The assembly of the mitoribosomal small subunit involves folding and modification of rRNA, and its association with mitoribosomal proteins. This process is assisted by a dynamic network of assembly factors. Conserved methyltransferases Mettl15 and Mettl17 act on the solvent-exposed surface of rRNA. Mettl15 is a class I SAM-dependent N4-methylcytidine (m4C) methyltransferase of bacterial origin that modifies the mtSSU rRNA at position C1486 (human numbering).

Using the data from recently published structures of mammalian pre-mitoribosomal intermediates, we analysed the T. brucei maps and identified a number of previously undescribed structural elements. First, we detected homologs of RbfA and Mettl15 (previously referred to as mt-SAF18 and mt-SAF14, respectively), both of which are associated with Mettl17 (mt-SAF1). Structurally, RbfA is anchored to the complex by its N-terminal extension, with the C-terminal domain binding Mettl17 and the C-terminal extension binding Mettl15. Together, these elements stabilize the subcomplex in a way that Mettl15 and Mettl17 form a heterodimer that is bound in the cleft between the head and body. In total there are 43 hydrogen bonds and ten salt bridges that stabilize the Mettl15-Mettl17 heterodimer, which contribute to two main interfaces. The second interface involves catalytic domains of both Mettl17 and Mettl15 (residues 484–512 and 176–198, respectively). These data suggest that in T. brucei Mettl15 and Mettl17 form a stable complex, which has not been observed in other species. In Mettl15, SAM is located 42 Å away from the methyltransferase target residue cytidine 582 (C582, equivalent of human C1486), implying a non-catalytic conformation. The Mettl15 conformation is different from that observed in the mammalian m4C1486-containing post-catalytic precursor, thus implying a pre-catalytic state. Finally, we identified 13 hammerhead-shaped densities ranging from 17 to 22 Å in length, coordinated by tryptophan residues within a helix-loop-helix motif of pentatricopeptide repeat (PPR) proteins, which likely represent cofactors such as acetyl coenzyme A (acetyl-CoA).

> MFLIHFVHYKTILQKYTFKFKHIFLSIDKYNSLFFNISGILIWLNIIHINIILIKYSFFILINNFEYLIILIST;> MFRLTAASQKNLNSWYTKGTMRGGVPRIYYAWMRPGSFTRRRFEKMRNPFVDLETGTSLYFRDTRDSAEAIAHAADSKGIKGMDNAIDLYNEYRIVPDLYPEGFQWKHKLNTEYNQWRSNTWLTPDLIPKEHRGRFLCNFQLNIVAYDMRVVKFSPKDHRQWIYCVLYVGSGKGIAGWGRAVAPSTQEAKKEAIREAFSNIIAVDLEQEGPMYPVRVNADGVRVLLYPARRIVANFRVADILCAFGFQHAGCRINLKATNNPKSPTHTVEGVFEAVKALRSVSEIAASRGKVPHSLIYNIYPYLEEIRRRKGMMAMHPPGKDGLLMPDRVVDNRLPDHLKKGYYDDVYWKDFFAGSDEHLNEPRMGLRGDEMRRRLEEAQTSPAPTTAKDTRRRTLEDVLKRLGKTTRDLGSIPIVNPRVDVGLPTHIKRNYQLH;> MVFYSFVLVMKPRQRRFTSQALREIGVAVYSNGGLIRSITNEGIMRPYSRFRDADNTPLTYARYIILQLDMGEEEMGKVDKIIREHQDVLMALKLNNLERPVGIRSGNKELQAAYFPLDTFTRLEEEINWSPQTSADIYTQLEMNWKEFSRTRWSSFLRN;> MLRQSLLSLAKVYGAVPPLGAAQGHRLLHGKREREGSLFAVANDVKRDERLLRQQLNALLEEERMPMQARLQRNEAVSSHEAVPQTPLVDLPGVERRRDLPADPITRLFFQHKGDHALYYGTYDKPSVQDDDRVQIEKRVPRRREENLYTPIYDFCHRIREATEQRKRFVVVPSTIETRGCARVMHDHGLVAGFRDFHNDRAFAVELKYFQGDSTINVIEPCSYDGRTEFEWSPKMMRRLLNTHGIHNRLVVYICRTADNRIIDHIHAVKENIGGRGLMMVH;> MQKLLSPRTARHARLFRLAGKLADSGSPGVPKSDGERLVWVNSHVRRDKDISLSQEEERIRELMMPLEVGENSFAANGQATHGNLFYFREYPMYPGEYVPAEHNTLSSLRDELRLDLTAQSLKEAWMRVSGGVYFQSVDEYYASVDGLDAEQIGEVLAALFPELNCYEAQALVQRTLECISRPVSAASRQLSRTITAEAVGLDNAPGHYTNFLEWMGRLTETRAFKTEHALFEFSRRKFNRDDVRVMFENYRLMSKATLLADSADSYSHFYTVLKDFARKVAGEDSRHQIGVRIDEAEVDPETGIAVGRGCADGEKYHFTALLRENRDHNGIITVMGKPLSLVLDNKAWLMEMVLMPFDEANLDYRDFDVHIVSEGHAMPSIANEIAAFALRMAVANALVKLIPLTRIPLKKSGLLSVDRRRERGQFPGYLDGKKVKRRFAKR;> MVRRSHVVAYYWSRYRMPTQMPKFDGPAPVAAPQSMNSTKTNEFIDPIDDKFPMSIRGPLVRPDVPEDQYVDSWYICTSMTHHMGDYRPWSASAPPNAFRFRPFNEFDAKGREYVQYMREFARFDPRKSRGNGQKGFPFRDAYLTKMNEANQKTPPPTLETIMDRAVREHHQHARILSPLEVQRDVGRLEPIPSYAGKINADRSVFPFQWKTEDWYEYEVAKVRNRRFVFENTEEDGIRGSEVTYKIVLEGFWDHHVMKLAEDVCMFLKDVGRQIVEEKLVAVRRLLQGGAVDPELLAAFNCARAGPFGGYDEYDKEEVANFLRSDLRRLEEQCLSVINRCNVPVPGATNIYDPHTSWPHVEKLEPWVRMAEFWTSSSDTSFTELEMSTAHYEFRKFFRVIICKLPFQSTEFEKRMYDIRHWLHRQTSCEFHTIYRRNVIHDSAVFPTEHDPATPTTHEHHRMFSFALDWQSAPVNRLSTDTVREGENWDAVAQRLGCSVGELKDANAERETIEAGVVINVPVTATRRLTSFGATPLVLPLKTTSAKDGERIRTWEEAAAILDCTVEELQQCNGHAALTYQKKESEAGEFDSSVTELVAPLSCWTSTSESEFSPVERVHANDTLVAIAKRLQCSEEALRAVNDGITDVSGLDFVRVPPEARRPRRLVEPQLRPQAATDALLARTIAEEETFKLKSIPHLPQNAERFPHEYHTPTSRFPPTPSETPATQDWMAYTAKYLDKQFTISAEPAPVYNVNKLWPMQQIPGKVDQTPFEEDQTWLLHSIPVQQLEMHHHEKDLQDLPFINHEQFPRSLEWNAP;> MMRKSVTFLRRGKPRPRAGMFPDKYRRVPMLLKPQQGGQQYFNHFLIRSTNDRLTQQDVDNASGQAHSFISPQLPQMDWRNMSARSSEESIREEMRQLAENDVMQHQRVFNERMWYEKEEEHRMKARSCPEETSEHAISNDGAVPPPRVLGGDYFKTRFGYSLVKNSEMTQGPVDYSQLDMWGEMPRYTSDMVFLYLVSRRRNTYAVAYTYEGKRILNTYTAGNRGLKGGDRGFRSEGSTDNGHQVTSMYLNDLLPKLREMRASEGRPMGRGEKVELVVRVMGFYNGRQGAVRAVQDRANEFHVRYFEDITPFPLNGPKMPRGVFK;> WMRHIGQDVPKRHTHFVLESRLMYEKSFRDCWLHSVCRAISQLDEPLSKTVVGTHQKMLQRKVTCFQYNQYGLFKTPYYRLANVDRYHAVQGVAGTREWVPYVNVSYWTMNKMVRGGNLLVHRVHYTGWGTDSHLKKGGWEHRWNKVLQRNVLQYSRI;> MFVRSFCFLRKYGSKSKTPDLKTSFTKTTNFRKAEKISITTTDGEIVKGRGKIRRRTHSALKEAIGAMEHPAIWLWYPWRMNPEPPTPHMPQRRALKNVHGAVFNDLTPVQKKRQEQMLYGVNIPETRQMKFEEQHPLLAGALRKLEGQPKGFPFWYRKYPTRRHAYEYRFSIPVEMLDGYNDDVKKALSKGMMSIQEKQFAQEAMYMERYAEHDFDTTSPAVLAVKRALKCRVLRNHLLTNPHNNIIKTVLANTERKLNHALRRLRKVDFKKYWEIIRDHDVQDILQPPNLVTYRQGSYWKYDWNAGLAISTNLADVMDPRGLNGCVETGRSRSEVARDLGLSYTRPLHENEKKQLSHQAVYYERLAKFKMEQPEAARAMERERFVRKFSGMFVKMDIRSGAPDFPSTYRRLLGTKVVRWASKRHGPN;> MQVTETVLARAVIKRRSPQLWGAPGAPIIRMRGHHVVWKFQSYDLVVEHTHKRRNSDIRLLHYLGKHCPHPQKSLWSPDTPVAQDRHLFMLTTVDIDAFKYWFGVKRCRLSMKPWALLAKAGLLPPSLTQNSKIMPKPLFDKESLMRYYLANRKDEDVMAREKYLNYENSMVKTEEERAAERPVAPYL;> MLRRSLLAFPWWNFQTEHRQRCVLMYGGARTKNTHNANHRVFIKKYKRNAFPNRTRHHWAVSMTGVLSQRPRRMPWPYDLTSLIFNQPRQGSDKIGYVVGTSMLKTAVVATNHMVYYPKFNQRVSRTKRFFAHDEDLACVEGDLVHIKQCRKISKYKHYYVFSILEPNVEGRERLKLGLKAVPPPLFGYPVSRRIVKLNLTSTEGTQEKLAAAIQEHVQDAYRFSGPTPDQPRNRLADPVTFEDANNMIAPNAPAAAALDASDSPPLLDRGEYTEVEQDTRNKKGDDYWMNLQPKEKYDFKSFKKSPRPLEDQVDPRLIDGKYDIPTTASENLYFQ;> MNRTGGSIYAHALSQFAVCRQPWNEYIGLLTKQDSTPYHTEPQEKPAYRGRKQGREGWLFGQQVQLHYHRFPDEQLITNLSRWRTGETVGDIAMQQFRNAQPFDIEDKDPQGVQRPSPEVYMKLNYKNPATISRFLTRTGHMYPADILPLNPEAVVKLRVAKAQAIRIGLYPRFGNPFWFRSQKFRPKAYQENYDPTTYSTKRTVEHFAYNWVQTDRIRRYFRELEAVHTSGSASARGSGGGTTAEHKQQDQFYSPENQPISLHRNNISYMEDVGRSVKNPTVPGLMSTKGMKKKFHNLYSSTSTKRMGFSNPTLGIKKV;> MAFRNTFTTPGKFSTVSKNIVLLLIWRVKVFLRAEGFAHSLVMLPVSLYSKILLCDVKKKIVYFHCCTRKKSMLRRCPCVWPDGPTKSSVSIGTAFTLQKRFLKIAKSAFGFYLARRGQRKYPFLRRPHIKNTHSMNPSAPYFWSFMTAKSQMAFLPEENYITGDWTGKFFVSKRQVYTLQHATSGAKVRVKSFPSIFEFNSPSRWNIGKEMNTLTKPRMDLIDEQMLTKKQRLDYVRAGLLPK;> MLRRAYIQRRYPFNKRGPREHKSWKHHVLTEPPKPLQWRDPKVWTRDLSVMKSFDAPQWDLWQSRPRSEDMDEALQPFMDMPKSLKDRRYDIPWWANPFGAWYLQNILSLELLKLKSKTNAEKIATYRSYMRSLASGKDNTMSDDDVIRNIIKERWKTLEFGDRNAGYPCTFGDYIQFLNEWFKSLDEEGMQRLREHFDRRIRPLLAVMSPVDILWLEALTQNSPHNKEQLQRKIAFQTSLGTPEFFDMSKRLRYEINEDYKVRDELGPELFALWSKAPERWPPERLSKMYGLDFTLVRKILVWHHFKACYDACVEPDWSLPKRLFALEWIRDVRARKHGLFYGKMRFAEQKITFYSDRFLFRDLVNRREASYANVWEMDDPYRFLQTEQDYEDYWGDNYDVYRRMFPEMIGRTGEPVQQYGQMPIWAGPHRQHANKSEHNWMFAEIGVNVGHEALKKLELDPTNEKRRRFVIRQPDGTLRSAKMSEMRAWYWKEEWADFRFWAPQMEWGIENTPSQEQYQEHVPDTTDADFRKQRRIQSRPVKWFYESHYTRTGSFAGFQPLRFMQRRTEREVRWPDVINAAVQIQKRKPAAYIFKAIPEL;> MRQCVVRRYKMPKNMGVAPRFDTWNEKYEPWEHMKRMGRLVGTGFYIPPEWYNHFRMFPPINHNFQQEKTLNPHNASEPTQDDTSTLSPERVALRDELARKSRLVASEGMRYYNIFWVRKPLDTMEKEYYELKRRGVDHGEAIRKVLQGFYSGLAVKKRVAAIQAEEAKLTGRFITMREATVVLGVLAKLHKEQLTPHQVSLLAKEQGETTQSGAKLTAIVSRTQPHVNKEASSPATSEAVGSSTEESLSADALASMLSEDGEQSAVGTRYQVEVKETANDSVRQLREKAEDQTGFPDWYTGESPTYSGTS;> MMRSSSFCRRQIRPYYNLPSKSEHGRKMTGFLTPYRHWMWKQNELWRNVHEAQFEHLRRVYKRQWLESFRVNADEYIYKYNITKAAQLAQWECEMKEQEKKRIEARQMMDGRQALKKKHLDLLREFHERQFFFWYERASERLQNMNLINYVPHAQLREHIDKELDKYVAGKNEPYPLNFVGQMPFLEDGDGNIVEVPESLLSNHMAEHPDSTAKPHEPHTSSSISEAAAFEERMLRAMVSAKEEDLKEWLGDDSRALSETIDDISREEEEREADIRVARSMEETDAEREVSRRAYIERGKTGSRSIFRPPTVSEGAGGTPSAPAGDANTPMRRRKKGKLDRVHALQAHQDELLAKLSSQGLKEGVDASSVPERGKIVQSRGRIRDKAVIPTHEVLMQKPELAAGSTPGARIQTKDMVDKMYHRGKYKKSGSGDKSDGEDL;> MRSKTLKKSLAAMYMRPPVTCYTDACEAPVAMWDGAIPLKETRKLKNGVPVRTVSRTYSHPPQLTPTQLSFNDINSMYCVGNDELIQFFPEGLGGRVFQTMPPGHPRGFLYRKETHLLNLFVDKVQHWHTKRSVLSSLTNGRTGFIVDGPTGCGKSALMCQVVHFARSRNIVTLYVPDAKVWTHGEWCWPSTILPGFFDAPDAARSFLKYFAVANRATLTSWKLRCTPKDLPTEQGERQPQNLYELCEWGHRAVAPASIDRQSVCVKFLMDELSEEKKLPVVIVVDGWNLFSHETHFRYPHPDFLRGLASFNESSTDIDLYPQELPRIPASRLSFVRGLNKMILSGDDPNKFFITCTTRDFKPFDGISGFPNVETDRFANSLDEYAPYDPEKDSHFHPIQIGNFDEYEYRSFLRFLINSGELAGLGWGPLWHASSDFERKLYKIGFLSGRNPQGVVDHYHQELVWRYDYQRTRQKQYLLKRRMEGMSRGA;> MVLRRWFPLLGVHRVGYTHPSTLPVPCAQRWDLRLARARIFQEYIEEKAPGAWQLEDERSMSPEFKTFTGYPMRDMRPGYGQNLPDYIMKKRLPNNTHYELFARRDIPNEDNAMYGKYLYDMTVHGTSLPSTYRMHKDINKAQRNDRKLSGNRFKVLCSSGAKNPPSGWEPIPDATEEEED;> MLRCARVALRADPLNGGSSMTLGSKGSKLSPEPHRRRMPWTAAKEYVPGVVLNARDKMVLDGVQLLDIESIDRASQLDPLEVLRAVVATREYNISTGKNIFQLASQATYNGRGQRFYRKEWQEGTYDKYVTLSAIDFDRDGNKGTAYGYITFHGETTTRPVQVDFADVPGWYMDFVEERAVPFTGIVPPPPSIGTDVPVDPHSYRLKAYPYYDAPNPPEFVERLLKDRGVLPDTPTETADVDKDPTTSDGSVHYDGK;> MRRWHRSLNPALFGERGSGHYFSTTRARLQLQAQDRIICGTHGAGIVAHQTAVNSSDNPMLSSVTTAAPAADLSRTKPHEGTGTSERDPYIRTLHNQRSAAPESSVSQSHTVNAPTVDECEMLAERWGTMNYWHNDTFPRLVVFLKKLLVPDVSPLSPTAESLLSMFEKVVIPKLTSDEEDRRKLVSLWSETTLQAEAAVTKFLFQRGSFESMLHRIITDALEKMSTLALGGQEGNLALEALKRQTLFKRNDFIQKRLIDVVSNSAYLGYGDSVWQVFFAAVEANEENLLSDRATTDAIRAAWEGVMREDVVRLPDVTGVVALYLTLVCIRESGRLVPEELKELSSGLEDGVRPGVRKLQQYPLIFLHPTVKRRFVVKAVAEILHNSSSNAFSNMLRENGLHDTAREVALCEAMNRNKELAEGDVGDAVGRFVSKGEVKTLLSSLVSGTDAVVRDAVAGIFGIGTTITIDWDAVMQNVDWSNNWQRLATALLSNSAVLSAIVKLVKNAIGAKGMSKHLFTDEYADQLQLILDAREERAASRKQRIENIAQELSSFERVDLSCDLLRKLGVDMTELDTAAAATRNMNVVQRPCIEDGLLSLVLEAVTKRHPNWVKAGVIQTTLKDPFDALRWMMHIFIRLSYVPHAGAATIARLSRRRIGPIGLEPHQFNVPAELGFVEQYDNLQYKRYDWQGWYQRMLDVHNRNVSLRCRICDLQRLDGNGVQFVDMQTERRLRILAQHRVGMGVLKLDADKYEDQADNVTFGTTKLSELLADARKAQLGEEYWPSVELKVRKPSGQSKAHYSLIDNERIEKRSRELYEKYRDAKKRSLFVTPMETWLEVKGMQVRKSVDNADEDGYTLDALQDMMDGDDGDKV;> MRAGCVACSRIPKLGIAALGSTTTSMQATCQETQELRCATTQMAPAVIFPLPPPLRGSYIDRKPTAASFNEHHATASFRHHMIASADVSHRPRHFYFASGTRNDTGTRSVKEGERKQLKQQTNVEVDSVAYGDQLDELSARWAAKFYGQVTFGPRNYPYPSSRWLARRFQMKKHRIIKRFRFRRYKLAAVANLPFAKMIRVGMLPELKSSKTKRGDVVDPTLSGQLVSAVKNTGEKRKGQRTRPKSKYQV;> MLKRTLTVLDQTYGPHKSYKYTYMPDPRKLAPIETTQRSEIVPQSIRPPTSYVPNHETFLERADIHRLRPTSDFKASFKDWNDLFTCDKRQLRVRGIPRMTRDAIRTAVQAFQNGNPPERFDTKEEWLYYKQFKTVDYSYRVIPELPEKYRPHQSGIDQAPLPDYREINKMPQWAECEERRQSKKTV;> MIRRRVCDGARLAPNIRATFSAARYQSGLHTFIRDSKPSNFSSVRRSENANGDATASPGATAGENPASSGDWASHMQRELFGEVDPLGGQAHKDYYRDVTRGYSPQYAPRNFANGGAVAYPHIQSPYEYEEAAHRRVWLDHDVDRMREEFTQHRASLRSLASAQEREELLRSRAAEYQVANTVHESESVHPIQQLYNSGGTSRSALKQQAVADRYSIAEQHSPLPLTTGVDRDALDEAQRTKDRILNDSFTAENLLITHGLREKEKHDFTILQRTVRIPFQGYDMDRFLAQQKGTPYGAQQLPPNVVPSSMEEAQRTLRGSSATATPLVDAVAQKVYARNTVVDRPAIGEQLTEQIINTMRASRTTAEQQREEERAQRFGLGRHGALVQDGGPDQRTLKKHINDERIVDAMLFQQNAYRKTPADEHWNPYIRRSTENGVGHLLQNKFDIMRREDRLSKGEQDLTERNTIHYGVPIQQIVDEFVFRHRNARGERPLDYFKPFPNFRALRLNRMYRDVEGFSLMKQRPEFLEWELFTRYRQHHQQRRRLALLHGLEPVANETAQERDTRRHRLDEICERTPFDEREMHVNDDEMKVSVETLRSWFGVYMLPSPTVVNAVLGGSASVNLHLYHLADEMGTADTREHVLSGRYLNRLLLLESYQNRVGRGFMNHVVGRAPEPVVPHEQPQEVLRHFSAEERAMYEQHVKEQTSRQLGEWERAMKRRRWLTDHQQYGHVVSHGLETSVVDLSHTETGAVLTVSTKAYEQEIEAVRMKTNATIKVDGMVYNLLPNSERRVVPLTVQLDSGEKIDMTSEDFDRCELEAFPRNLNHALNYGIANYAYNRGNYVETQDSIWEEQTASGQEGWSPATHADGLREGLPVRARRPIFSSSAEQRIAGGPQRAVIIQYHHQPFFNPEPRLVKVAFQCDGTIMEVPISDVMIWQRRYHGPERTVGDESRRYNPAAMRRYVDVTDPFNEKTSNTEHFLDKYEPKRNADTVADKYRTTKQITEIDKWTRYDSARADNYRPLSISHRRDYIRMGYIPRYTPWEWIAIQEADQPLIAEQIRQDNIGTSYFFSLNRYWRYKASPHGYIRHFENEVRDLLQYVDGVTPWKQAQKIRTYWEVRSHHPMPQFNRPEVAMHRNTVGLLPAHMWETDKKTGKVKSVKDSVRDYQTKTPYPKWVQL;> MFRVRRLAGFIQCSPCGKMGPLKQQTRRYTPIWKSDPAVDNVAPLRDEDERRTLWAEVGPISDVGSAVTAWIRFGNDPVLHTAVPTMLGGKFRNQQREKESLLPNSSSPFAYVEDYMGTNLVFGSPVHAKESAAVWATYFERRYASRLRLSRRTVANYVGLINSPEVFDDESDRPETRWSQDTFFRECAYLSEKFLKEKVSNMQQFEAALKRASPEAYLAFFDAFQQQTQTQIPLPSPSVWHYEGERRKQWAEKFISISHKAQAFFKDVLSEDVKKYQEVPGKLLQKVKPVLADVGKILVKRHERWLKGRVWTSLTEEEREAYCMKEVKRQQMQVEDGEFDPMMEDDVDDTELEEWQREHDAIMELMNSPIDGLHFTTLELWLHAMRCEELETEHIYTSARVRAVQVAARKKLYDTTSYEEVIQAVVESIARGTLDLGAGVLRPHFNEVWCQLNYAKFGSSTITQHTTTSRRQLLFFHAGSLKDIAATATLYYATKPLSNSLDYASPYKYRRSLITLCSNYGVETAYTTQRPLLRSAANLARAEDLIHAVVTAAAQPFGERRRAATRDLHMEFQRLAVPVERVIVANPVSALLESGADPDEKPVEGEKVNMWPLGAKRVVLYKWSAPNVEKLKAMESDAAPAVSGSSLTAERLREIQELKRRGFLEVSLWRRVTAQERKQRNEIVEAKKKQVEEVVRTVPSLAHLHQYATSLYSRIEERVAFPTETSTVTDTTNMKEETNKPLEDSEWEFAVLLDDRVLLNKEESVELYLPYRDANGELLAQGEYRALVRAFDLEANPNLHPAYCSVGYSESFHVFDALPQLIAQFFRVKDATAEAAGVTHIPAADFTPFCAFLRDAGLDVPLRCEFEAGQAVTTDGDVYMDYFLQLLRGEAFHQSHAQAGLTEAQRAIEPLCRAHWVVHHPGADESEWATARRSVLDHAMQHEREWWFPNEMLDVKDVVTGSTNGLTPQMYPAAVRYGVELCTVLTAEGKFVDERGSGLSARCVVNGTGAAESVVFDTANCNGTNTTSVEDALRVAHGALRSAQDRHNTLAAFRLGPLSKQSQVLLFCGVNAYEFGGKYARTYAYAFEKAKKELEVTAASGFMAPSLSHEDIERLSDQPTTSPSVDRFASTTHPEQRKAQFVPRVGPGSTPLEDPAADQKSEWS;> MLRCTVVGHHRSGKARAFVFRDPSLRMMRAGSGYQQLRRMGMPMQVGMGWRKVDSFHANTQYQHAWPLLSHDDLGNSDQSNNTKNIMYSMYMPKRNKGTAPWFRGADTYSVKYCEQGRYEYQRYLMINRFPSEYKKHFLSFLSNIRMSSGSATIPQEALHWLLRMIVDNFNPQHVHYIAAMKTLQSAGELDMARDVWKIMERQQTWPCTATICAYLDVCVEAGEKTWAMEAWNRYCTELKFLEPGEVDPKPISRVPFSLTREELLYLPKWKKHFDHDPNLDVMDLNRFNRTREVYLRMAQVMLAGGERNAFQHFFTKLEEAMLNKPTPVPEPPNPHLVRRPRWAPYEHCKSVHHSPWRLQNNGRALALGPSVTIEDEMQSRFFSNDQFLVHSVKEVLRIVLQEHKRAHPTECTRCKTEAFFYKTKDADETLKFCDDLIERLFASLGVRLSNLNTSSLLSTILEVFRVVGKESGAALLQRANEFLERKASLGDAEGSRENLTASNYLQVLSGFADESAFVYNTKKDGTCQYKTGFDPRTTMRHLADVVQEIAGNPHVTWAADMHLQVVETMVGCGTMKANDYFVRNVLRQFSWDSRFLEVLYVEYRRQDDVDMWAELTKRALVWTARYNAPASERLRRLIEDDYDTIRVQTRTFRELAVFQFRDVEERRHSRDVVNELPNPWYDYVAHALPFPDRDAGYPDEYGDLGQWRAPGGPGSPVRGPGYYAPPMEGEHQRGYTAEWRDLRNPMRPPEFPTPWERKYRQYARGQHPSYDMVYAGPMPEIFPMRRDFRKPTRWDFHDIEKQGKYRTSGPY;> MRRCSFASTCRYRSADDVPLGLGSAYVWTCRNITSRGQFNPIHNFSYAMERGVRARDVKAFEKLITNPGPLRVAYTPDYLDWLHRCYKAKGTYMDARAVAEKKFNGNIVSSELSAAVNRREGKRGDTRGDTVDNDHHNLPGAPPPGMFLRPAHSFRRLAGELKRRRAQSILDEVARAQGMLDLFERQPHFPAIHIDRCSRFHLVELFKEMVLERSLDSNMIWEKALLYRAILSERKPSYPTSFHYIFTAVEDTVFAPTISTPMEMAGSGGEGHDRSSHPLAAKCPTLEAYYYYVYLVKKYYIDNAVEAHVVLRCHREPNAADLLFSNPPPKDDTEIMKAVELLRNADIQRGVAAAAAVSDPTLPPGGEGSVIGNSDNKKNSEKTSEGSRGRPARPPVLPGAYPPIDMLWRCEENLPLLKVLLFGEFNLIVSENPFVKFPSAHGFLTRPYSTDSSRTLADGMSLANVMAEKRGHLLPSLPRNTATSIDARAQDIRRLQQKHHRDDIVSFQKLLRSTHAEDSPSAFSSYSDWSYFNPRAVRAEERDRLTRKAVEALKLYDSATNDIYRHSFEDVQACHTQRVTERDRTMPPYLPTLPHFVAIIKKDPHISFLLHIGLPDRNSSEEGSAKHKELEKRIYYLARALYHTALEYHNETVRRVNRQKVNVAASLLDNFVEQEWTTILRDKHDVTDVTKTLNDTQNDKKQLARRLGRYMLFANRSLDDTGFPTDARADDYTRWMAPPSVGKVSL;> MSVSGVFSKGRGIGHEAATSILRYIPRARVPWQPSRFGRENLTAADMARLWSRGRYRDGPGNYNSGYCTERTHVLEENTVSIIPRRELEKYMPDITIGPKALVTPVSLMNARNGHRVTHDLLHSYDPHIGRLGKPAVVDHDNITVEDPNRVGLNAATLDCRGRIYRWLRRGPFFQVDNYFRRSVKLNRDGTLPTDFVHEAPLMRKIIRLAHRGHLKAACEEYRRVTTVPPVEVYRALTACCVPGAKLADAVSIFEDGNSKLFYVSRDGEVLHNLMRCAIAARHRARIMWVYNVMRGRFYENVVVRAEVDLIWRYRIAMIALEYLLDHECAEEAAAIYSYLVEEELLRCDVHVRVGLHMREAIAAGKPITLNDDVMNATSLVRDATAVAPEVARELQRRHAQTLQNSAVEAVGAENVREGSAPWSILGPLTAIGPTAEDTMVWLQQHYGDVDVMSIMRWARFRKGKDLMAKDRPQYLARAAAWIELLSKRNREMEEVPLTYMRKSKPLVLGTNSNVRVAWQTPLMRSGGPPRLLAREEGYVFHHSNSSRFVEETYRHPGESLQSRYLALQPLHTEVSVKEDFQRLYYQAQKHHKQQERLLPVSTAAIPSRIVHHSVMSALHGVSGKGEPANRSLFTGNRSNDSHSNTGVASGTSACTDGAGSATPEF;> MFRRAIPLLSANIPRSVWDPAQHNPNWSDSYGHDITNRRAWPARKWTVGLEPCTPREWLQFSHRNLAYAYNGALRACHSLPSMLLLYKEMKQRGVKVDVDTMNVLLTRAARHEHIQVDDVFLLFDELVALGARPDLAAAETLHTVLSHSASMPEEWREARRLQLVELYNNLAMEEVERLAPHRADRLLKEQMKRFRGNLQQLGSGLRPTVYCRYLHTTHTAAVLLEEVHNFLWELVPNDHPAMEIPALQLRVPFVASVLRRPSVNPGVSLASVSRAEFGDTDVCAVFLAAAERMVDADFDDQRPVSERRLFLSLLTMISYSGVLYTSDLMAQLMEMVKYSNNDETRDSDAQRVLRYALRGSSAAQDSASRTLWHSVEKVADCRVVGRYIGARNPWNPIRVCFDEQGVFKAYPISTTTTTREVSPPEGNGAVTQEQRASCVEGRTLEALNMRWDDVRRLIECTGVLVTPPSERCPQQQKMEVFTGMAVYLRTVATGRRYEGGEDVLSDGAVATSSCEQRRRGTLFAEGYDFDVWVRLFSLVQEVRHDMEKFMADHTLQCVEPEFECWEALLVTLRCALDFCVVQMQGGGARGTEREVVERLFRDVVALREELIEESRTRFGGRMRVLWLQEA;> MLSQNVAKTTVPSYYMIRTNLPHRKPQNQWEGVYYYSGITKRQRHLILLHRKREREAHMRSFNISRASVLQRLEQLSGDRKQESLPPHVRLDLAVRLAQHGLYQQATPIVDELHHQKALHAGHYALLINALACPRLGQRILHCDAQCDPALTYKLLGDENGEERAQEAYRWFDLALTSLAVDCGGRTQPSQFVRYLPQGTAAASHITNALMRTLLTCGYTHVAAIPDSVYDRMGSMGISPTISTYELVMLALSLQGNMVEAESILSFLRSHHSEHITVESFNALLLGHREARQFDCCDAIWQELVDRRWPRASPLTAELYLRSIMDHANTPTSEPLQSFANINVVEKKKVPLVLAQMDELGVPRTHLSRVLMDEVEDSLRKFQTYRSRFYEWGRAVKQFDFIEFRRRNGWLYDLHLMKCTTKQVGPLRDFNDPDAVQGAVATAEIPAFFNERPAWERPPLEETLYVTTNKERYDDVRGGDIYYDDTRSLHDRSPTWMNEVPETRYDRLYGVNHPDIAKIGIRRHLNVEYVNRKEVVERDAALMKKTLSSGRRLRHRVESSRTHRNAGSLSGISSTAGGGSR;> MRKFCHFMANCWNSARSHATYGAVPLTHSQVTSVYATDGGKVDELGLLELVEERIFSWKLNKWEMRIPPNLPNDQKELIRQEQENLKQILSGWRKCFGALNADILQISSLTGVPKEVVREKNRTWLQEEVAKLRWMGEVNKAALLRDAFMRLEAFGSRDFMFMERLCCIYGLARQGTFDEAFTNYITEDPVTNDIFVDERNPFKELVAHIVRNYSQIDIIYDFLGFNYSEGYRSSLRRYMEYLQCKTAENVRASGRLVTGDKGEHNILFDYCVSRESLVSGDSCQGIIDFLYINGNDVTLIIIASDNPWLRNRQLPHRRQMEGIARRVCFVLGIPPSEVRIRNLLLPPTYLDKGSIVRLNDIVFRLSNEQSNLLIPWLTNYNKELDPKDVDYTALAKTTNEEEWLTL;> MFRSTRPRSVGYTPVNPDTSPMVAYSQYHWHYNLPQGMERPHSVNRTFAAPFQSNHSLVNKYRGVWIEFDMHPAFSVALEPQLRKLPRGRTLPKTPAEEVIADYTALAPLVDDEKTRDLWLAKVFQHCAFQRCGGAMELWERYCHQRFTAEGATAKPPLSLVKSVLFYCNKTDNSGWRALFDRCLKDGWNYTPLFDTAQWSFMLKSIGRMGDEDGVRAVLEEMLDVQADLDRVEARSVVIALNAVTNADVYEFVKKYLFNFGERKVKFLRTTYSDLRGHGAGKLRIPLKENDNMYYHVCWHSSIRSPRQFSPRQLYFDYTPSTLGSSSHNPNAKIDDIVKDKIEKWKAEGLLPEDYVHEDRVYDRSAAFKNVARQEKWKKMPKILKSKRMGYTGDP;> MSFRYTNNLIGALKHRLLLESSYREIASRKFIGNCRGVEVVCSGYGTVLAVQLTDKAVWEPFYRKGGRPTVSGGGDVSGDAETGTQGSATTTGATGSLDLDKLAESIKTALWDATRKIRSAKEAALHRSLSHNTRMRASADLKHWYEEDANTLRPLAFEALKHEAATPWMQLVQHGKKEEAAALLKEFEQKGDAAEATPTRVKDDRVKGTRTELSNREQPPLASTLKAEDSNPATIPIGSVHPLFTPALVQIEEAGSGSVSNEAVCRAQLWELSRDEQLFWERVELIRKGQVASIGSSHKRGYADEAAFAKDDTEEKVQLRFTQ;> MRCSCAFLDKSVFAAKRRVIVPIHPTPNFPAHFIKSAFTTDPLKEKQKARFSSGGEAMREVQDIPKNLEGERSRRDLASRGDTEFQALVEFIEGASYDQLISGRRFKKVYDVLSENDDMFIWLCHTAMSVLNPGDMRSRLIYNHLRILAESVASGEMTQRTAFRFFESAVRSPAYREIAKRQLEGGAATRLAGISAAADVMRRMGLTRRPMSSYFELYQRIVERSEAMTPWGFPPLFQFEERLSLEPRLKFFSRASQQSLERRRRGHVMTPHTTLHGRRIFWIPPTWNRAGRFLGPHVTLYPGMTPD;> MRRFCTARVSSYVKRAPLLLPRGGRRWRSGAGTTADGGGEKEYIADSFESTAGSNAYAAMELAAEARREIHELWLSAETALEREKRVQQVAALIEKYKLDPSTPREADVSRGLGDAFDRLLLLCLPLGKTDAKGTDNLERLMHLAGRNGRELSVRTIQHLFARTDSFAEALAVFYTMRRCHVAMNMEAYYSMLYSLQRLEEEGWGQHFRNEYEENGAPSEQAMDFIVKGISNALLPENKPWLGRVMFQDRNVPDRRYDTRDFDELDTAWTQRYKSGTPAGAH;> MLHGTPVRRASLRYRRPYWMMFLKGVDNWKIYTVIQQPDHQRTEMLYQAWLGGLDRPYTRPKCMANQPLWLSKKRHMLRKERLDGPETPLEKYVLEWHKKFHSFQGTERPTPDDLHTALDLVERPLDLSYALQLLGQCRNLNNIRFAKETFLVFLEACLRVGRRDCAEYALEHAEPLGFWFIDEDHRRYLQGEQTWYKLSPLDNLYYPVEENAKLNEGRKPITRLSPATESPGSGTAISDGEPSTDVEGETTVDDEIAQLEAELAALEREGGGK;> MFSESLCILSRRFRYNTKFPALVSYNKLPWEVVNHETPQFHMHVAPHYEQLLTLAASSPVPHIISSKHIDVPREHRLRLLPGMLYLLDGDTLPEEFTINRVLDPTALQYYGRLSSQIVTVEAVRMLVSDDLRLLCNCITFKGPLHLPVAPYASLASLRGASQGGTTGSETGSNCFTLYHFVRPNRPPKELQLEKYYIHAPCVAPLSEFASNSDERGNWRPRLQAPKRTQRATPLPAYRPPQSYLMGLAERLAVVPGGCFGRRSLMWGHWF;> MLVSYLRLQADRRTRHHMMVDGQINPREWFNWHPKEYQPWYFDRHKFLYEQRQYAQFHHLLCHQVYLKDMLHLMRYPEPYTHIIDCRTSTQKMHRWVPHSLWLPRDEVEYALQLSADEFLDMYGFRKPDKSDDVILLSHNGIYSEQAGWEWKKQFFQHVYNYRGGTNELFGESYSDMNVSDVLSPWKGPFPQSGVFVDKWSKRKVLTRTGPFDRQYEMQDFALPDLELEKARHPEEGPRQNMPFGLQ;> MRRGALSLLKAGLLGHYQQEAFEARKRFEESTTYPGPIRAATPGDTRFYSGSLESILHDTDRHYWRAVTDDPRVQHLIPLRIRFKIFTWVTSGWEQRMQVVQIMAPKDSTIAQVKDLVLVENQSPYLCVSSFHLAIDGKELDPQKTLGEYGVTEQSQIDAIEQNDHLLHRDDERPRDWTVDEITAEDVKRSPYKEMEMQPLQNLAPRYEARPKGYFGRTYYSGMKQSS;> MRRVRDGLFLSHPSSALQCSVAVVSTGEFDHPPFQFRQRHTFNTTPLHDANRFGGRTAYLREIGPVNIKKQGRRFKKDPRTVQFNVDVWCAQQTLRKRWKQRDWEVIEIPFRLVPREQQRVIPELYTDIPQMTDPARNDFSNIRNKVYDREELQGVLFPAAGTMLYPPLQRVDKQAMTLDKYL;> MLRFTHRALTATPERFSVLGTTHPKPKRTGFGRNNKMRSKPSDNVAWYDKGPVEWLPRPVRLTYDHLDQLQQWMMRATLDGRTEEFNRIRDLHREWSQHPLMPVLGDVEPKFPLNLFKQNHRAKKRFLVRWHKANTPANWLWMPRGPTVVTPLHRTNPTQYPENWKQMVQRKSGTGTPS;> MFHRAFVSSSDLTGCTIALSSVCTQKRYWAKPKKRPKVGQGFHEKAQKWREEYLLDRHRALADSLRAYVEFSTSKRVEPWDARFKPFDRIEKDGVYVLMRYMMEEKLQLCNYHHRPVKRLFCNIGLMGPQITTKARWKPYRFATNPAGTSKAERMYQRDKTVYTHGHND;> MLRSTLTSLNTFLTSSVATPPISVIRTGPKWWADPERMVRQKLMYFTLGVDQLPLRRTAVIQRDLQRFHMCKPPPRVGDSTGYKRSRAAQLNTWYRRIQYQEYHMQHLFTRHVWGLLRVYPGNTTKIQGKADDGYVGYDSVPFHRYNRAPLPFPARELYERRK;> MLRRSILFRMKYADLELTTRGEFPHGMKEPAFVKKLDQNIPWYFSTYRSMYHWPITGDNWSDLNEAEKHHDLHMFYTLAWWKLGEGIFGVDEDS;> MFFRFHSTTLQTCLTSGVARSSVAVAVPLRAGCTRREMSSGGDGVLEGAMHKPGESGLQAGSSTTIAGKETWSQFSTKMRYGRRRIRVIDVAAKMSYEYQMLRKMCKRRPAMRQWAVRDDFCDMNPGVVIMSPSMQAAFMKVFRMKEKGLIRQCLRDIVPVIEYRNREEPARLPTNPADMIPEGEPDTLNQKKRELFERREKGENFADLRLHDKRSQAKLRFRIRQRLLKFQRQLAVANAIASRSVLYSTNDAIGYFLFRGAAMYAGMHRVFFELSKQLPHFVPKTMLDFGAGTGTAILVAKEVYDPGSLAYPLYRSLRQTMQGNDSSRTHQLSELRYDLKRLQRNNEEKKKVRFMAVAALLERGEVDPADLPEDLKREIAEVATAAATAKKDRLVREAHARYRDVVDGTEWESGDPLGEVRASTEDPEDVIDGEQGDGGDDGEAAKGRPKTWWEKLIDVENETARTRAARRLRPLQEVTAVEPSPGMMEIGTMVLHDDVPNVTWKRYLLPEDEAIQHDLVVAAYSLSEIATSENRRRIVQQLWKMTKGVLVFVEFANLNNFNILMEARDWILEEKDVGLWDWQPTIVAPCPHEHRCPLRHCKTGVKRKRMRICSTEAHYRSTFVEVWARHMPLKVGIEPISYLILARNELVPERAERRREQLKKAEEMKRRERDVKQQQLHEASLAVKDVVFERLSDEALHRVQSSVPQPLTDIDEVREASTSATSTSLLKDLKDGATSTGEIGHMPTDVPRLVKTGNTRHNRLIFPLQFPPATHKFNRAFVDAGYQRQRAITPAEMLVVRQEVEQLQQRVMRAAPKYLRVVRDPRCHGKVQADFCTPEGDLVSGRVYRRFYGDRNRVSAHSTMRWQHIGGWKLLKRIRRGSLFPHNVPLYAVTKHAQIDFPNTLLDTKHSTVEQTAMQYNDPMSLVEMPDDGLTREELKQKRRLQRDVELQKKVEEKLEDIFGVNAKDWKTDDLGGGRLDARREISEQQWADAVRRAKIRTVQHTKNALPFAAKKRAAQRALQVRRRNVRLEMSGNRRR;> MLTPTRRLPKALSPYAQALRHVALRGATAFGPGAKEMELDMLRKGTLPADYRPPVQGRWDDTIERWAYAWQFPAEEEQDDITKSVERNASGMQALLEIGNKLLRSPPSPEPLSGKASKLYPPVGDMSSGNTALLPPNPTYDVLEQDVSELMAEDAVVVASQPRLRAEELSAKYNVPMAYIDDSSEASNASKSLALVMEDVGLEFTEDGLTVVISALSRQGYGTIGRAIFDFASTMGLGPSAEMYKALMKYASRRGDVNESMALIEEMKGNGITPRIGNWHELMYTFYKAKDYPAVSQIVDNMKMYANIEPNEVTFVLQLKALAKDNSQLNSLPEAIQLFDQMENVYGFIASRPHYDAMMFHLSQSPRPEMRLRCEELAHKMELMGIVWNANTYLNLIRSAQVVGDVAAVEKYLSRMREEGIPASIGHLTWAVQAHVQSMIRIDYDALKEKDESPLPTWLEHLETCFGIYELVVRRGWVMQLPFVNALLRLTCQATILSMERTPDEAETIGRFEEQANKIWNHTFDEWQLQKDVYSYECYIALLAHQQRIDEAEKLFQEMILKKDLSPSRRTYHCMIFMHLSSGEEGGTARALRYLEAMERAGIQVRPSLLKKIVRVNNAAGYKRDMKRRARRIMQAREEYLARKAEGVSFGEGGKEGASNQRADVDAEGNSILEPLAVSPTSTLAWWEKWKRETVSKHELFTEEGADGTPKGETFEEKNEALRMMGITSSFQTKDLVPQPDRQKLLPLIRREEGEIAGSLWAMDGGELSYPKDGGGPQGWGVRLWRERQLVKREYQKVLDGYRPVPQLSTLGNSVRTAGDQLDIERSGAQTPGELSDYRNFPDNRFDGGQLKPESEAAPAVPFSAELVWQGEANDKLSPYKSDEEIALENDNTFFSSLSKETEGKLSIAVKAMQNKEENSVDVRGKGVTRRSKFDYLEKWRDMYRHGTLEVPEGPTLNFGRTPDDHKETMAALVRGWYQRNRKEPASEEELKRWRVDEQRSSETSASRAALKKRKQVRSRHRNK;> MLRGWHPNSSAMQVGMRHITIGGRHSRGGFRQPLGKHPQVKQGTVEGVPRRIPGTTKVTYTNKKGRTFSFSVPVSELTHPQVTLESAAGTWREMDTSFCELGDIEDDMPSPVDECLRGGSSLDKRLIQEVRERFVSFCREYVLMDTSGMKSTILSTELNAGPDYEHYDRRLRRKRHWLAIRHRFEDVRYVIWPDVVEETARGDSAQADVSLTNPSLTAGEMLEALLWLDAASTFCVRKVHPSDLGDKSEFLPLDLQREVEVVACHARRDLDFFDPSATSLEQFTACAALCVNHRVPFSLFFPAQDVCGDASVSTGQCIVANAPSPHTALGAVRIMALISEGSGSDIGKTIMFSDAFGAVTRFGILRGLSRVMSVEAFGCKDALENVNESELCIILHFCAEVREQNAAFFRRYEASEEDSDPQQVSFLAKYQQLSQIALARCKRLLYHPDSPRAQVMSEDGYIPLVELQRHAEGTNKAALIHYNLGIRSAQGMRRVALGAQSSARLAELVSRLEEASARVSGNTLVNDLVHHLSHKAAAGKMSLTLREVNTLLPLLSRMRRESPNGALDARFDRVFNAIDTAIGAAMRHNCTLDELLDLAEGLAACEMVPSALKQVEMVLIRSVMMHECSPMHLRRMLQAMFTLMRTSVPQVLLQSVASRVADYIKEASHMDSSSSNGGGDEKVKNHEECEQLLELLVVLGKCGYGALPGLVTIYWEAQLIDSMQLNPRLRCSYASLLASAAFALKKHDKRAWEGLADESHRLFMEYTRCNKENDIGRFAECVTGLAVLTQIKDNTNSSDVAFLKEYLSATSLELKSCEVIRVQELTDLLGRTLEWSEALGVVAPDVVIQLEKALFVMLENVSHTAPGVGIPDELVTAACCLVDMSSASLELRKAAAGVVGGAIVHAEEALETLRSGAPTQVRPGHSFDVAALASAERENVYKNSILQYCAALQRSGMSTHVEELWS;> MRIATSPTGRGKNSSVLPLLRRFSWGNGMCSPYYTEHRRQSTLTSSALSSPANHNQQVVYRSIRDCRERAFHLIQELVSSPIPGCGLSYSTNGSFGGPSLTVNAVSGVASLLELYDKAYYFLHLLHRTILVPRNVVRDTDDFTEFLLRCFRRPSDSLLKGDEELQMSDTAIVDGFVEWMETSLMSAGQFVSFVEVLQLVGSYVRYHKGVRWGARPSEEEWYRCGYRLHPWHDTYCPSSRAEQMPYVHLLQWLMRAKPTKLEEKIDDKEGAHGASSLFSTAAKESAMRAWYATEEFSPPSWHTVVGNSNRLGFTALDCGCHSGYMTELLLKAGAQEVLGVDVSPHHLGNAEATLSEHLRERRSSSYSRKTVQFVRCDILPDLPDEARQTKTPPLGPEGSTNSAAAENRRRLARCHHMPSDSDGLKTETEVTGPFDLLLFHPPLPLLFPTWPLFHDLYESVDQLAYDAGRRHPHCRLSVLNEFLQRLLGSSNGEENNSERRRNAHQQLNHQRRLVAPLIKDNGYVAFILPRNFDTRAILQRMSTSSAGKNCTSCGSDGLAPLVPLSDVVTMTLEGSYTLVLKRSHSLSSLLNRMDYIQKSISAFIRAFVSPQHRSRVEQEVRDFYSNHQAIDLIVMRKIARQKTNEDNDNKDCSVRAVLQKVSEPIAYEDSFEYEEYIPAGGSPLAHHWTEMTPSFSYLEDEFFGCADSVGTNGPPNGASFLAVGHPLVPVTRQLVGVDRFGAGGRDATQGESGSFDKMFAKEMRRRGGRMRKMALTPLEKQEWYIDEKLVKSEAAKVDLMNELSRFELKDFD;> MRHTIPFFRRSAFVPAPGSSLLNPRSQRAKVRRMVAAQKAQGENFERQALYAELGGSPSARAPRSKGERSKEATRRVGCEVAERAKHMTDAEWEGVPVDEKHAFAKYMHKVLQEHPTETTEQQRRRYFETTMADVFELDPRKTVRDEYERVKLGLPVHLKNPQYSLGVSQAVYDAADASLFDPENVHRLENAMTHVKQVFADYVHKKREGVSTEAERRMLANLTAELNLETQKHLANMFKYAEMRLRQVKLEERHHQLAEIERLRRMAQQRGGVKGRKGGSRKMSRMERLKRVINRAVGLDIAVAETVLTEMQAQEEFLQFCEVFARLTLGSGFKHTGKDENLSAYIESLRKLYSMDAATLSTLDVVQYYSSKEGAHPVDWAKRWYERALLLPLQSTPEYQKLLQIQQRDESTVKHIKETAGTGHAFACEAEAEVARIKTQKVVNLVEKMFMDPKDKRLESLHEKRLRYLAHMQMERQIRCVRENAKLFDGVENMPEAAQCRELYEKIMEKKTAQCNMTSPPEGEGSAIQSAKTEGDHCEVGPGMFNVYDDAEASSLFEKIREITLRVIRDRHVQSAAATKARMLNRIIRSLKGGEQSIAEELRALHQQRKEKMTMRILGIIENDVKTEMEWLQNMEEAERPPLLPIPENMSYVSAADVQAWRELREDDERKAANPFERRRRTFQPELLGQAWSVPNKPLLFWGTGVSAVQQALRHVAEDAERKRQGLLLAPPYPCAENPWGWRLAKDILDDNN;> MYKKALHSFFLKVHPDFFHHNRSQQTVNESSVARLNELLSWAKAFKSGHLQPPPSSSFTLTFYRKPDDNMGNGETRREGSGSPVSSLVGRSMGDGSLSPTIIQSTFELPSNFAPSDNHRGTVERAVNKFLRDLLRRAACIDSVTESISEAEDATAARAEAKPLRRRPRGSQHRGAPTGPKSLLDEAVESMTVQWSLTPAPTLQELIEADQILFSRDLSPLQSAAALSTLQRHLGELNYSAWESMPVIVSNQFSIGDLTGTITIPWDFTPEQFHSFMAHNEKGVARCREVAIQYASTIEQLIAELCTALELDDILVSCSHQDALRLMELLHRNRELLIQYGLSKLTLEVGNRHATRANGVVIINCSLTSEQLRPWLKAISPKLPLQQRLYELSKQMLESTLWHLKEFRTMVEPGGVDAFSNDCTYAERLQWSKELFRIGPSLAPWDWSEMTFVLSPDVDIDWANGLLALPYNFDGDALVRYVEEVQQEAKSRKREELLAASAMQREEEERRRKQQHDEELMVECQEKGERSGDDSPTVAERMRHLYRQTNPHMDEYLASSNSRVDTLPVERPLSHAVTFNSDAEAEDQLKWEGFYAEPYVDQAPTSDIDDMAHTFMLTNRWHREEAAKKMLDQLRGTYGKKSRRFEYQKMGDVLEINNAKVQPKGFPTLTRGIKPGC;> MLSHAVPRLRLAAAAVKAAEWYAAENRRKQKGGDVTREKVDCTAPLWFDDTEQNLLAREQHVRSPAYRELHRPALTNAAMGLYGGEPGFEKAHRVWVDPDRPHIKHIYNQTALARNLRYARYGYFKRDMHLLDVDKLVRHARLLPTPGRLLTDFLYQRVPLPDKSCAALIRYQRQQIEMLEVWGRHASFQCAVEMFERMIVTNIPPVEVGVETHGEMVLCAAACGKWEEGWNVYANRARELEKESPESFILNTFFFDALLTLCVAAGRVSEGIDTLEEVIKRNLRPRGTMLNKAMILYSILGEQMSKHEASRATSEGERSYLCEPEEVEKMGLEVWSLFDFYQLPRTTASIEAYMRMCCAFNKPTLVLKAQGFADASDIRLSIECFHWLVYAIRGVAGFGDYVMDVLSQLRPRGLTPDFVLFTLSFMYCALQRDGELALAIFDQHFVHQNMNPTPEMVLLFIQACSNCEKPTAAMLERSETLIKRLEAVGSSVDLISPIYDQFLELCAHLGAVASGFSALKRIVGFGKPLTTRMINSLLLANSNAISSNGSLSMTEELVGFFTLLKIRPNADTEICVNLCRDAFGESPVVNDFIKVIGESLQGDSEKGEAPQYDEDIPVIQVPPHELRQLRTEWKLSPRDIVLRRFGQHTKPPGKAALDVGSMRGSVIPFGRSPGEQLV;> MMHRTAARLRMPRKPTPYVRKFLEGCPLPETLVDDIAGANLKSMAPFFTTAPRYIVAAESRLSKLFFHHALYPAGGARRPCRVLIVRGGRSVREPSFTINTGGGRGEVGGGSRGYRDPARRAYFYARPSTVGPFYSGNGGVSSNVAKCHSGVGSEGAGLVKRASVDGLLSPLCGVIEAHFAVGGTCNDAVATEGDGTESLAKGGEKLCATLAGLLSGGHGGLMMDDGNCASNVRAAKRVARLLHDAAHHLSSFFYVHTQLPDSALFVSGPEASIASNGKGDGLLPSHLAREKDNDGRPSVEGVAVFRLAGGLEPTVHFAVGAPLSVLQRGVDGTASRGEKNSAEEGLNSAASTTVLPFGHIQCLLRVRTRGGKHCAVGKEGSEGASNTPWCNTAGNDDITSNFAASGPQIAGGIVEPWKLGVSLDPKVPFFMRTLTEKRPSFSCGEGNLGTCSRSGDVDGNTVNDVSSSSGGSRTRAPGEVHMNQLLVRNDCETYLLPQRELLLSFHVPEEAEAMCKEQNEERMRRQAALGYGSPSHVFAEGPRTFARVLHGMKANLAAVEEASSTFRQGAAEGISPQVNGGSTTSGSSRVYEVRALPGDVVFVPRGWKYSVERIVGTAIIDAVAASTASPREALRAVFRTAPDPPLPQDVVRCDEGHAGAGEMPGGDSGNAEIVGVEVDAFVLCYKPYPVLSNAQASTYVAANYVHSGIDDFYAKGGNDVYHKYT;> MTGPTRALFLSSGINLGRLRLAEQFSSMNGWQSKEDPAFDAYVKERRRKENYEAFDQRVERGYAAAAKLHKAEIQNAVKRRLKSSGAKFTAETLREMSSAVTERLAWLRDVWAQIDSDYRSGDSARQETAAQEISAALRGEPNDHMRWVYETKRELRFAGPVGRRAIQEELQAAELPEVLDEEVNRYHDLKLNMMEIEREVKAKYGVAGQQHWAELQAAKDEEYIQKLDEAAEVYKQLLDQSARLDESRRSELQRSYVERVHQAQVRFKAAMELEGQREQLIEAHQAMKEERMRTEREKRRQLLREAAELRAQGKESADVLTALKERQLDANAKRQAEYELKECEDILKRKSEMLDMIAHFKHDVEEREGREMLQRQKSDEERQVNVFGFYEEVGVEDGLSISSEGTTSQGVSSGLGTVSTSTSCAKSADSNSSAQPSQKLRKEELWKAINADTYEDPFRTVHQARLDAVKTYDPAYARTFPLNLVLGRKYSRQGAGEMAAGNETDKQILQKGNNILYSFQWGLNNGTVHDLDADGSTDYFMDGAFHVRDKETGDIDWRYEKKRGGPVFRGPKFYRLGAQREAADPGERAMDPTPYTSTPREHKWRSS;> MPSASSGYTFADFLRRLERSPDSHMAPLYHEHRELFVRRHDMFARVISSVTWSKGVALVAAAGYTQAVNVTIYRALLARMLLHNRHVRQCGAGSVVPWSAALRTYSEAIATHGNAVPTRMTLSALRLCTPARQWVAAISLLMLSQANDKLTLPMLIDAAGCCATPAAWEKAMTLLGRFHAQSLQVLPDSIQSLRPVGTSASTVDAAAHALLPRSEGPTPEQKHILTVINKVVSAVPWQVALSNEMCRSYLTHLVASTTLRPTEKTASLTTAVQQLPWEAFVTLMKTVTATVQEGSQGVLGSRSTPQLPPPQDGMERGDVAKSLLSNSIIREGVNLLQSEPETAIPFITTILHKLPSAEAAALFLSEATSAYRNSSSAVVAAAIRHPVVVGALLKRCADSNSWYLAASIFKSTSPTAIPCDVASDLVIQMRRANQAPLVVDVLQKYIVPSRTKLTEEAIEAALLCVLVHNRALAKASAVVAGTSPDNRTGKPNGIGVANGVHWISALSWATDLLEEGVESRILQTGTTPSVGGVNHEDPTVLLRKKTLSPRILSLLIYICVNAGSPRGGLFALGYARTVSKTELELSEEITALLYCMMYDRPREAESIIQHAVKKHGEYKGKYLGRLLVASQEAKGSALRNQT;>[2x]MFVTSQLTHMRRLSVSFLPFHLIVTTQRRQFGGNSKDGHKGEDKPIERVGGVPPTGPHPFNITSGAEGQISNQQRKAHDAITQLFRDDAQRKALYQKPGRTIGAQTTTAAISTPPNEDEFEGLQPISGDAEPSSITAVEAVEQELLDDAFLYFPPAQQSASGSVATTATNELYVPGQQIIPPGLTRYRVDVQYQGNDFDGWWKSTTRQLFRREVGLDGSITRVPVAEPGTIGNAAGVSRGETMGSRYHARTVLEEALAVALDVNTVRVVAGVIPEVGVSVRRLCCHVDVPSHIELQPRTVIQRATMWMEKRQQPLAILSYRRCKNQDFHARHSGLRRVYVYRILNRVAPPLFDAGLQWHVDRHLDVDRMKRFAKTLEGTKDFGYFADPKMANALRRAAMSPGGFSTGAVTEENFQPKATGESHRVTRGKAPKVTMEKGPSNLDRAAALPTFNEYGQRVVQPGAHGKEYYRVATNLPTVRTVDRLDVVRQDDEVLIWFVGRSFLRHQIRNMVSVLKAAGHGLWNDLELQQALQSGFEPSRHRFKRERFPTAPAYGLTLWDVEYPDQHRDDYVQFVDSGPYEQVNIARDI;> MLIRRLRRPHSTVRGCRISSASNSDSAGAFSANGTQLPDPPYYLPHSPRFDAERCGTFNKKWLLNLPALKPLVRNSTYLPKKEELWRAPTHEALETIIGHLPYHDALRYITEHSLFLLFPTVLRARDAPLPHVIYEDFMKSCTFASLQNPPEEQFALPSVLLRTLLCMAAYHCTLDADYFTTCQMLFGRMEQQQQTTPEVLSAWVYCCTASGRVDEALTYAKYMADCSAPFDVTVFSLMQHPSLNPIEVEDGSVPHSAKGLLLQRRLGNRLHTAYRSDAVAAHGMFVYYALTLSHVRKWEVIRAAAALGVTLAERTVVLAVEVFAREKGMRCGPKTVKALTHFLAQDGTVGHLLYVLLRARKNELLPEFRDLPHTTFSEEEQELVLQCVAQRARHDDSFAVAATLVSSLVREDDPSELLMAFARAARNHHSADVCGGDGDGSVCADVPAPVPESPPSNSSEIIEKDRWAVVQASVRSLLLDVNALDQASRRDAYHKHWKNGNKGVKNKENVLAKTLTLPHDSMHTATIQRKEKELWELMRSDTPVGVRELAQLNIMEELQEAKRLERAEMAWVNPDGTF;> MKRYRSSVVTRLVRAITLRPDATVDPERYPLGYVPLDGSESVDSVWSLVKSGAFVAPLSKIETIHRAHVGIRYLTQSEYPALSSIDVVGLQTRLKELCSRLLIRRDFWVLDDYNDPELNSSFGIQNMYFDNFKWSQVLWRRFQQYVEEYFPVAEHTHLTYDEYLQLLRSFSHFEQGAKLLPLLPKRYRIHPPFGVPALSRIDMEPLLLYSQWLKNFRGPLKLDAALVIRSGCGAAVFATKLNGVPIVRGVDPNPRAVMSCRKDAQRMGRRFDSISFRVGEMFPDKDDGNGVPNSRKYDIIVFYPDQGCYNLFFTNAIGEYAPVLTGFAGTLEHFFEEAGDYLSDSGVIVLCCTNVYSILKPTEPHPIEYEIKVNRRWVLLDYYDMPVRGKGTLSHTPTDHHYRIPMEMRKCMRSELWVLHKMTSIAHFAHIHNIPGAQPPSCVVSHWRNKAIGKLRRAVLKGQVESSGGDWDDYKKRLVHLLQEQSENDEDDKAQAIRMAMDPNYPKELADRARAAIEKNMDTDKAFHNNVAKAFGDISPRERFDAYLSCYRL;> MKRIVVPHRWSEMNRVEHPPLMMKQLFQGVCGGLRWLETKSLAQYLAVRAIEEGYPSTPGVRKALHVKRAPLQKRRVVQRSTKSATAACSLPTTAAPAQLPLTSSGDALTVTGGLSLQVTKQKRLVSYDVLDCTLGSGYHAGAVLENGGPYTRVVALDCDHDAMHAARDLVEEFGGDRFRFYCCKMSEAKAMFGERSFDAIMIDGGVSDTQLEDPERGFLLDDEGGHRLDMRFGPQMGVGALEYLNTVSQHTLVSSLLAYGLLEYGQAMKMSRAITRRKPFVDSREVLTCIEQAGDELPEGGWRSQGSRRKSPMSWKFLTSLRCIINNEMYELRQGIENALLMLRDDGRLVVFSRLPWEERLVRGTVDDHPHALLSYVEDISIDDVQIYGFTRHAKMWVITRAASSAYALKNTTTLTEEKFRESSVRWLTGMYAGQTHGFPANNFTFENFERKEWVTLRRNGKPPPVDVGLDDK;> MRWSAVLCKVSKVPTRSVIPADALRYHPRYSVPRKMVLSNTFNVVGENNRYTSLKLILEKLSGHVGRRQYKMLCNLEKHYDKLKDEGIDWHELKWLSREELIVLFDKVLHLTRTERAALLPAIEAKVCGVLRQTDSRHSTVVCMNRGNANHGWRCGRNGHTNDVYFEGKAKANTAALQLCRRSSVRSVERSGVLVEVRSEPDFSVVGRFDHSLSPRVWSTPENPTFQVTTIGYEFRVHQEDPRVIPQIVEAAEEWELHANITKQVIWEMLEMYAVERDRQPLDLKPGEMGDPDIPSRHATAFNVQVVPPLSEGDEAIQVVEQRIVRADGSEVPWFQEPPPQLFSGGIPVILPFAPSIIVKSTFRQVTRSSAQDVTRQLLQPVVDVTCFLHPNVCFWWNAEDEQRCLGHIVDYAKRIPFALPFNLYFRVNLSKDLRGVQNYTEELGKRMSMKAHYFNLRSYGVR;> MLVCCRSSLSLLARATMPLCCSRRFLTHQNNIDDISGPVDTNSNSVSDGRLHCSTGEGGKASTCERVSLRTIAESLGAAAAAELRAEVERDTRDGVAAIPPLPPLGWRVRHPSGSNYFVMTRTLKNGVQSAELNNRRYRSVHDIFLQSLQKGGHKYAQKGKGSEGRQKDAKEEEEPPSQEDGKSSPKVTVGYDREGRGHRATLQRMDELHDSPKLSRADVHLTVFAPFRVYDPSLHDPTVDICEWSSFDLVVQKTVPDNMVANKLLQPLSCTPQDGALSMYVCLASVNSEMRIRSIQLLSMKEAQALVEHACFGNGEPLFLELLRRRGRRRPLVERRFDDPRLRYEEVAQPQQVADEAAVACSSSCYGPYYPAFEMLMDSCGSAGEYSRALCYGGPYVSELSRELCDALLDYIKGDLGVSDQLCEYVCQMQFFLEQEEYMTWLGQVQHVANAVSRTA;> MQRTLRSAARRKWGQKTWSPTATNGGAAPANGVSAQEALQIAYRPMPPSQTVEYEEDFGHNLMIHREYISKRCRDRVSFELSALSYSNLELRRGQEHLAGIMNRERRGVSVGASGAPDDQVQMQTDVDANSREVLSARYLFNERRLQFCDRFQNFFQSKLENSAASDSNGHEKQHLFSLMEACAVIFGCETEAARETYYRMFLGLDSETLLEEDEALRNRIADAKLVQRVLENNKGRQEVTQSPKLQQQQDQGKPLHAVSSGTSLLNDCEEERFISSIPELSLFEDETEARANGFVEGEDDVKANNGDLTAGSFSSPASSVNLPEEFEEYAPLYKAYITHAVGKGPVASYDISTLGSTGLTAERRRWRTLMEKIVREDYHTMTEVEQMDAIVLNEQLHTVKFFDLKIGDAIRDILQLLQRETGVGSSVNRDTPVGISPNNPERRV;> MLCHNRLLLVNKQTQKYRTKLRYRFRQPSVVPLRQTLQQRHNTILEVLRRRRINSGDQSPYRYVEERLYSKPSRLDREGVKVNKTYALQGLGDLEPLRYGANFGISEKDALKYETVAEKAKYMEPPIPYSSLAARKLAAGALWPAAPDPEGMISKEVRLLRHESSMSPSARAFSERVAYHLRRSLKACPGHIAEHIDFTQLIIQEVLGSRRSKEIYIVWFTVDPGARFELEPRLHQLNHWVQQLIIKRVKRRPHIPRVTWIYDGGRLERELPRDVKQELQSFVADAATTLESRVKYLKELDTMNQRMKDIPWFMPYLWSKEEKAARQKSMLADLEEVERRKNEHSSGRSAPPRMSPPPQFVR;> MHSSLIILRHAYFSALHPARRVVPGSLLPVRTQFYTRHFTSTAGPTCGDGGETYKSEPTKVGASVEGTNSGNGVTDSPSLFSSSAPTVRRRALPPSDFPENALLKCIEKEIEDEALRLDKEECPPPPPTGWEMYHAPGTSVFYGRRWWLPATASAETRATPERHTIRVQLTKRDPSLDPECDVRGEHFPFSFFVQRAPSKGEAVRRDGTFRMGDSAAAGDVKGRTEGKEEEEEEEELGLYDQSIEVRADFVDGELLVDNVVFHGTFKTGSSCSKRSGNTSPEAAAATAAGQHDNTTGGRGKVEEVRYNNIFNGYPGPNLDEAEEEVLDGLQAWLAERCVDDQFGEFVGQYSVWVEQQEYEMWLKRLRDFVAA;> MRHFRLNRCSYTPNLTSLTNQVNRSERLRKWGSVGVPPGFPRIPRLEAKGIAILHESPKVILAGRSRCNNFDSNQYMLINKATKRCLLVDASDDWPDDWAAFIGASDLTLTHVFLTHCHIDNIINLNAFLTICGSRQKQRVQVDSQDNDNREDDNGSDEIGVMWCPAEECWVQNFKRSCERYGRFEEMHQVLPMMCRSLYTPQHLVDPVIAGFSRRNARHLRRNDVLLSAATNRATSFIDFGNGVLLYYIFSPGHSPGHMMLHIPTERILFSGDLLFFNKVGRVDLPWATGVRLAESLRLLEALPDNTVVVPGHGRMTTLGRERRENEALQQCYQRQEIGKQEVSVGFNEGYL;>[2x]MSAIKRSLNVGVVGMGNMGVPIARNLGFKARSAMYLQIHSRALSKAKRVCDDLSVDGATCAMRIHDRYSTMTKWCDVIVLALADVKASRHALLEDNESLIMNARKGQIIVDHTTVDAETSRECAHEAARRGAYFLDAPMSGSPRACFNGQLLLMVGGDAETFQKMLPIFHMYADNVFHMGESGSGTAAKMISQALVASHNAAAAEALSMAHALGIEDQSKLVQVLDASWGSSTMLRRNAPLLQDLIRNPDKTPPTSAVSVDRLLSDLAHLDASLPKRGGEDEPFPVFDAALRSLAAASDAGMGDRDLASVVHYIEAGEAELRNRTHVPLGGEHLTGRTAATAANSSVNETPSTVNGSSEVPNEFGVEDFY;> MTDPVRRDPTEFLRVLRRMSRTTSWQKTMLFASKGRMVGYRLTREHYNTVLFSQSLWGRALEIVRVVRAMQEDKVQPNGATYYYIVNGMGNADHGWNYDFRINRRLEKIQHWRVALEALEACEANGFDSTDTMHNSALITLVIPGFNRWQQASLLLQRMLREDRRMHPTMVKFYHDCLVRNNRPREASSLMRLAAERGVHGYEDKWEADVYKGRPLDSEVMNESEGNGLRRQASSLAFASLMLRGDQRPLPENLQALLEEETTRNIEAERSVPVPFSAGLHATEINSVFRPRVYRQLWYKWQHIANRYRPTAALKRRQLAPRDSPTGIPGFYRI;> MVAKLQHNPAPTTLNFYEKSFQQLSDVQQRQTGLLIGAAVGDAAARALDGYTAEEVAAVAAESGSLQDEDEDPVVFASVTPREHKSGLLRHHSYTFYLFSQLLRVMATSRGDFPVQYVKNEWVATARAHPDCFVREHASLLHVLCITMQLPVIYPWADDSTLREYASDFLEFLTETPAERAVASREDVYAYTNSVLGVALRCLQSNPDPYRNAAFMAAPGTAHVFPDDLALYCPPALVGSSHSRTEELSEADSKTVPLFPARLLESDVRVVRECLVVARGAASFAEGIKAAIHLGGPVCQRSLIVGALLGARMGVRRIPISWLSATYDHVPLVTLALQVAQWSWNPPHH;>[5x]MRFINQAASDRAVINAGGRRFETLFSTLHRYPDTPFAQLFPLPGRGARQHRGREFFLDVTPHVFEYILGFLRTNQLNLPAENLQIRAEVVYSMNQWGLLEHAFPPEVIEDGEGCSTGGAVVKLPDVCVVQVCDHMQHDQGVKRHALTITYGADGFQLRSLIRRVRRDLERQLSSTYWQCYQTNERAAFFVTTKVANGTADLLTTSVTQQLVEHTESMGYSLASSYVTLSPDVVHTSVRMLIHNFTFRRSRRVEVEPGDGIALGEGSETIEAEPNIPTMHVGPRREPLNAAESIPPRNERAVNIWTVD;> MMKRTILQRCIQNKSLEIARISRSDINSRAHLPFNFDVCYELGSREFTLFSSVGSTSVLVFCNVSSRRLRSVKGGQGETEFPPKRLNVKRRRQSGSADRSPVVFSAFVSMPTSGLTIEALCCSSLGLLVVDGVSFHQGPLTESMIPQDAHPGPEGHYQGPLLNQRSLAEMVVNTRGCITSVDPFRQQESFFDGHVNPWNARSLRFGHVPVHTAKPGFSDALCHFLEVFGVNDELAFFVEDFAHLVHREEETAWTNVLKTMMGGR;> MSTSSRGILIAGLTNRARTQMAEGILRRLTAGTIFIKSGGVHHESTIHPLAVKVMKDIGIDISKQSVTSLEAARRQQNTYDVYISIDCSYERRTLDKSQPPRAEVRRRESFTVEYGDDGSGPRGGDDPVRYDPLLVPRTPSHWSVGVDATDVRRRWQIWSPRDPSIFHETSTRKFQDHLYEGEPLFMQLRQCPWRTQAKVSERWEMDEVAIRYPVERHSAHELRFVQAREQLLQRSFDLLTKLEKHYGERLLLDRALLEEFIS;> MHPRLSGQGVFPRYGGGWMHQFGHVYALQQELLNAEANNWFRAMELWHTARHEGVAMNVSHYTNILRQCVPPTAWEASLMVLKQMRRENIRPDVVGVGCALAACADANRSEEVEKVFSCFSGKLKLDSICYLALIKAKMSRGGYAEALAVGREQDADGVPFLPHTYTHLLEAAEVADDGEMALELARRMSSEQWPVSDRGREALKKLSTRHHWEEVAEYKQFVAVEDHKLSLPPTLPRG;> MWRLSRSLRSNSLHNPGPFLDGALQLIKLHLAHKNAAADKNTKACSDIEGEFLRELEAFRPCFTMSSSLKVAKLYTKKLHGALSYFQLYDDPLMRQLDMIIGKQTMQPSAGRQHGVFKAPVAARLDPFFSLDEREETVLPSELPNPPKPDPSTPLRERALKVPAQHRGHWVLRDPDIAITREERRTDPW;> MRRKTTLNIGQVICFSSWNDGSEGYEWKSRALSEKRSLALEFLGNVNKRVSIHDAIRLKADINKKAISNVSCPSFFSGIEGADEDEDQSDMSLCSLLGVLEGEIETDCITHLSPSDASLLKEEFLCDYDPSDTKRMAKWVNLRSETSDYQSYGAIPEGERSLWSAWYLRNIKAGKKPI;> MPPNSATRWLPFVSSDLKDYLNRYWAVMFTVGARPIETGHIRHYVSWYCTRMKVVLLDHHVYVEPLRQQLQEVSRTPELPLLFVNKKLVGTLRDVELLEREKKLKDVLHFGFEWRVGGSVAATNGQKSLMGALPAPYGDAEFFRGRYRGPPVARPVVSLPTLHPFALRSEE;> MNCSSTLACHAVVSAPSTASLITSCWTPQQHCYRQLMKSLRAAYFHDRSKLFWSRHRVLVEFYKYSEEANEEAVKQLVAIGLEVAAFIDHHMRTDVERIVKHNETMMALPVAQAKKFRSDYLLAEKQHDSWCKQKIKNIMKRRPPPPYPFF;> MQRSQLARKFATQVGAYSLLRGRCHAVSTWKVMATQAVTIPMYLPVRFHSEGHAAGEEAGRTGQYLLNKDDVLTRVLEVVKNFEKVDASKVTPQSHFVNDLGLNSLDVVEVVFAIEQEFILDIPDHDAEKIQSITDAVEYISQNPMAK;> MRHFGPSIAHFPLSANQLRFKASHIRIANRKRVEMFVAKRFHLPTRLATAAPDIAAEWHDELNPMHMYPAIIGIGHVQPVWWKCAICSHSYQMSVEKRVVRGGGCPQCVVNGKRAVADGALEGEMDSQLRPKRPVMFNMRTKY;> MSRSTVFGPGSLYSFTKFGSFNRSPTNCTLNKRMKDIFRLENQKHIRNDFDRERRYRMCTKCGITTVTINFNNVPSARVGLWGRCADDKDYTHHRMVDITQREYEVLRESPVEKRLNWWRYER;> MRGSLPLLFNPVLPPSTARLRLLTYPMALAQPHASVPLIQPTIDGTHDGRNGATVSLRTQARMHGTADSTMATAGDSSQNNSVMDSPRWLRNPDELCVAALRRSRDVNKINSYVATYKFDDPQWAPLLLPEVTLRPQVNSTGDKPNGGNEAAADVVSVGPSVSATPESTPPPPPSSSSSSPYSCHADCVSISHNKMIMLECMSRHVNFSLRHIVQKGHGIYLIYHAQHSILQPKGLVEQSFVTCSFGIRGERLRTDIVHVGPIDAADVMELQPSEGHDHPRCCFNLYQKSDVRRGVIAVSQVEGYGTWFQRKPMLWQRSRRIGALQSQLGAFAYDLVDPHEVGKWRDCEVSLLAPHMRFFRNGLNGAEAVGIIASSQVAQQRRLYLGEFEAPAITALDAVQQLAHASALRCKLVTPVVDPNGVGGTGSGSLGDENMDKHIDMETLLPLSWATRTPPPYVPLEADLPFKLQMSRPTVFAESHQQNQAYPTGGTVGSPFVRGAPMMMFEYNMHQGVDHYVYDDAPSARPMKWWSQKSNMPYSGYMYFARSGLVDRFTPSEDIPNPLEPTSKRKPLHAVVPPTKVVQERLRKYRRKQQEGHKQRRRASSGSGVSNEPDAVNRQESVSRGTCE>GSHMLETEEEEEEGAGATLSRGPAFPGMGSEELRLASFYDWPLTAEVPPELLAAAGFFHTGHQDKVRCFFCYGGLQSWKRGDD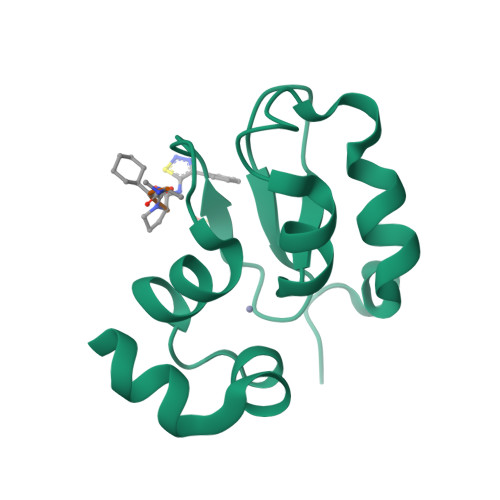PWTEHAKWFPGCQFLLRSKGQEYINNIHLTHSL[2x]>[4x]GAMALVDGFLELERSSGKLEWS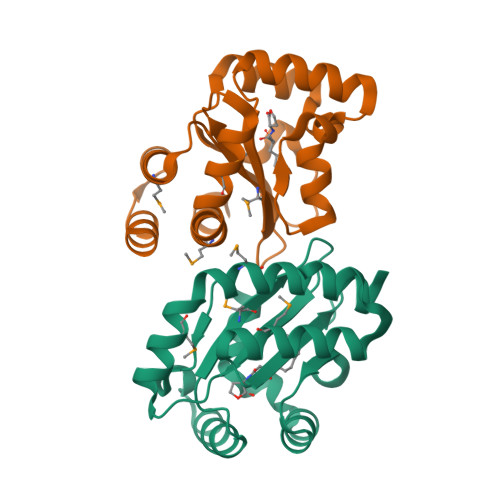AILQKMASDLGFSKILFGLLPKDSQDYENAFIVGNYPAAWREHYDRAGYARVDPTVSHCTQSVLPIFWEPSIYQTRKQHEFFEEASAAGLVYGLTMPLHGARGELGALSLSVEAENRAEANRFMESVLPTLWMLKDYALQSGAGLAFEHPVSK[(1~{S},2~{R},3~{R},4~{S},5~{R})-2-(hydroxymethyl)-3,4,5,6-tetrakis(oxidanyl)cyclohexyl] hydrogen sulfate 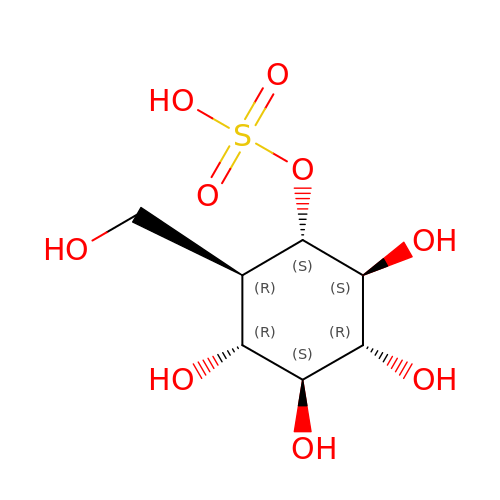| C7 H14 O9 S | PDBNIRCVRHFXAD-XZAJRHLXSA-N> MSSNRVLDLFKPFESFLPEVIAPERKVPYNQKLIWTGVSLLIFLILGQIPLYGIVSSETSDPLYWLRAMLASNRGTLLELGVSPIITSSLIFQFLQGTQLLQIRPESKQDRELFQIAQKVCAIILILGQALVVVMTGNYGAPSDLGLPICLLLIFQLMFASLIVMLLDELLSKGYGLGSGISLFIATNIAEQIFWRAFAPTTVNSGRGKEFEGAVIAFFHLLAVRKDKKRALVEAFYRTNLPNMFQVLMTVAIFLFVLYLQGFRYELPIRSTKVRGQIGIYPIKLFYTSNTPIILQSALTSNIFLISQILFQKYPTNPLIRLIGVWGIRPGTQGPQMALSGLAYYIQPLMSLSEALLDPIKTIVYITFVLGSCAVFSKTWIEISGTSPRDIAKQFKDQGMVINGKRETSIYRELKKIIPTAAAFGGATIGALSVGSDLLGTLGSG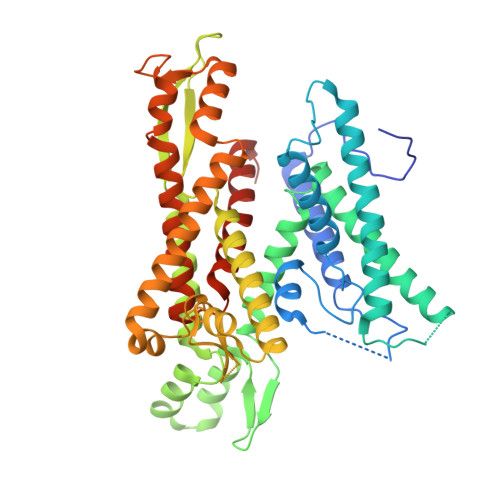ASILLATTTIYGYYEAAAKEGGFTKNLVPGFSDLM> MAGTGHTPEEALALLKRGAEEIVPEEELLAKLKEGRPLTVKLGADPTRPDLHLGHAVVLRKMRQFQELGHKVVLIIGDFTGMIGDPSGRSKTRPPLTLEETRENAKTYVAQAGKILRQEPHLFELRYNSEWLEGLTFKEVVRLTSLMTVAQMLEREDFKKRYEAGIPISLHELLYPFAQAYDSVAIRADVEMGGTDQRFNLLVGREVQRAYGQSPQVCFLMPLLVGLDGREKMSKSLDNYIGLTEPPEAMFKKLMRVPDPLLPSYFRLLTDLEEEEIEALLKAGPVPAHRVLARLLTAAYALPQIPPRIDRAFYESLGYAWEAFGRDKEAGPEEVRRAEA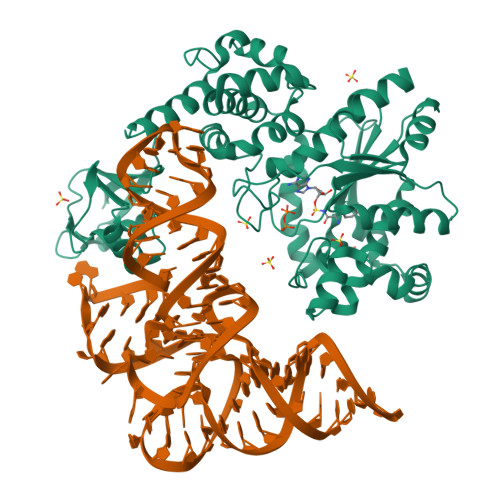RYDEVAKGGIPEEIPEVTIPASELKEGRIWVARLFTLAGLTPSNAEARRLIQNRGLRLDGEVLTDPMLQVDLSRPRILQRGKDRFVRVRLSD> MSKNRSSLQSGPLNSELLEEQKQEIYEAFSLFDMNNDGFLDYHELKVAMKALGFELPKREILDLIDEYDSEGRHLMKYDDFYIVMGEKILKRDPLDEIKRAFQLFDDDHTGKISIKNLRRVAKELGETLTDEELRAMIEEFDLDGDGEINENEFIAICTDS;> GSEANYRKDFIDTMTRELYDAFLHERLYLIYMDSRAELKRNSTLKKKFFEKWQAS;> MTMDTAQLKSQIQQYLVESGNYELISNELKARLLQEGWVDKVKDLTKSEMNINESTNFTQILSTVEPKALEMVSDSTRETVLKQIREFLEEIVDTQ

The yeast Sac3:Cdc31:Sus1:Thp1 (TREX-2) complex facilitates the repositioning and association of actively transcribing genes with nuclear pores (NPCs)—“gene gating”—that is central to integrating transcription, processing, and mRNA nuclear export. Sac3 is the central component of TREX-2 and contains a conserved Sac3/germinal center-associated nuclear protein (GANP) domain, which, along with the short N domain, binds both Mex67:Mtr2 and Thp1, a factor involved in transcription elongation. A region within the Sac3 C region (Sac3CID) binds Sus1 and the calmodulin-like protein, Cdc31 (Fischer et al., 2004). Sus1 is also a component of SAGA, a large complex involved in chromatin remodeling and transcription activation.

Crystals were obtained of Sac3 residues 723–805 and 753–805 complexed with both Cdc31 and Sus1. The crystals obtained with Sac3723–805 had a pseudotranslation in which one half of the asymmetric unit was shifted by close to half the unit cell, which makes structure solution more difficult because this effect greatly reduces the intensity of half of the reflections and so reduces the amount of data available. Therefore, we first solved the structure of the crystals formed with Sac3753–805. Three different crystal forms of Sac3753–805 complexed with full-length Cdc31 and Sus1 were obtained by vapor diffusion. The structure of each crystal form was solved using a combination of molecular replacement and SAR (Se-Met) phasing. The model based on the 2.5 Å resolution P21 native data was refined to an R factor of 18.8% (Rfree 23.5%) with excellent geometry and contained Cdc31 residues 9–161, Sac3 residues 753–805 and Sus1 residues 6–95. The N domain (residues 18–91) had the “closed” conformation (see Yap et al., 1999) and the C-terminal domain (residues 95–158) the “open” conformation, similar to that observed for Cdc31 bound to Sfi1 (Li et al., 2006). The Sac3:Cdc31 interaction interface involved primarily the C-terminal domain (EF hands III and IV, residues 95–158) of Cdc31, with fewer contacts observed between Sac3 and the N-terminal domain of Cdc31 than were seen with the Sfi1:Cdc31 interaction (Li et al., 2006). Sac3 Trp802 appeared to be central to the interaction and becomes buried in a hydrophobic cavity in the Cdc31 C-terminal domain formed by the side chains of Phe105, Met137, Ile138, Phe141, Ile149, and Ile157. The Sus1 fold was based on five α helices (helix α1 residues 8–19; helix α2 residues 21–36; helix α3 residues 38–49; helix α4 residues 58–70; and helix α5 residues 75–92), separated by flexible regions of varying size, that were arranged into an antiparallel hairpin structure that curved around the Sac3 helix.>[2x]MVADANGSSSSSFNFLIYGKTGWIGGLLGKLCEAQGITYTYGSGRLQDRQSIVADIESVKPSHVFNAAGVTGRPNVDWCESHKVETIRTNVAGTLTLADICREKGLVLINYATGCIFEYDSGHPLGSGIGFKEEDTPNFTGSF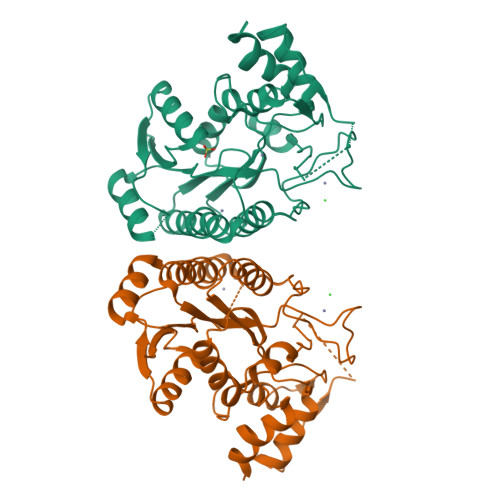YSKTKAMVEELLKNYENVCTLRVRMPISSDLTNPRNFITKIARYEKVVDIPNSMTILDELLPISIEMAKRNLTGIYNFTNPGVVSHNEILEMYRDYIDPSFTWKNFTLEEQAKVIVAPRSNNELDATKLKTEFPELMSIKESLIKFVFEPNKKTEVKA> HSTAETTLDSFFSRAGLVGEIDLPLKGTTNPNGYANWDIDITGYAQMRRKVELFTYMRFDAEFTFVACTPTGEVVPQLLQYMFVPPGAPKPDSRESLAWQTATNPSVFVKLSDPPAQVSVPFMSPASAYQWFYDGYPTFGEHKQEKDLEYGAMPNNMMGTFSVRTVGTSKSKYPLVVRIYMRMKHVRAWIPRPMRNQNYLFKANPNYAGNSIKPTGASRTAITTL;> VAQLTIGNSTITTQEAANIIVGYGEWPSYCSDSDATAVDKPTRPDVS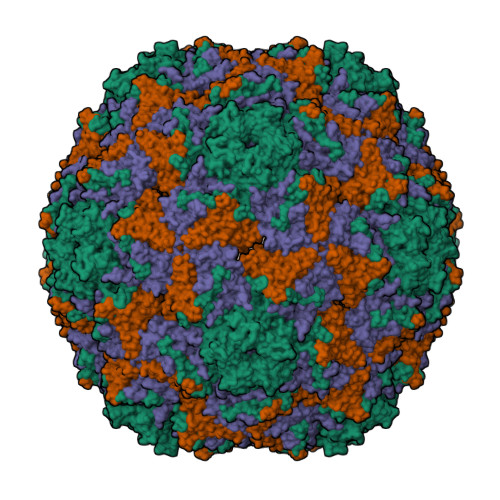VNRFYTLDTKLWEKSSKGWYWKFPDVLTETGVFGQNAQFHYLYRSGFCIHVQCNASKFHQGALLVAVLPEYVIGTVAGGTGTEDTHPPYKQTQPGADGFELQHPYVLDAGIPISQLTVCPHQWINLRTNNCATIIVPYINALPFDSALNHCNFGLLVVPISPLDYDQGATPVIPITITLAPMCSEFAGLR;> GFPTELKPGTNQFLTTDDGVSAPILPNFHPTPCIHIPGEVRNLLELCQVETILEVNNVPTNATSLMERLRFPVSAQAGKGELCAVFRADPGRNGPWQSTLLGQLCGYYTQWSGSLEVTFMFTGSFMATGKMLIAYTPPGGPLPKDRATAMLGTHVIWDFGLQSSVTLVIPWISNTHYRAHARDGVFDYYTTGLVSIWYQTNYVVPIGAPNTAYIIALAAAQKNFTMKLCKDASDILQTG> SPMSATALLQKA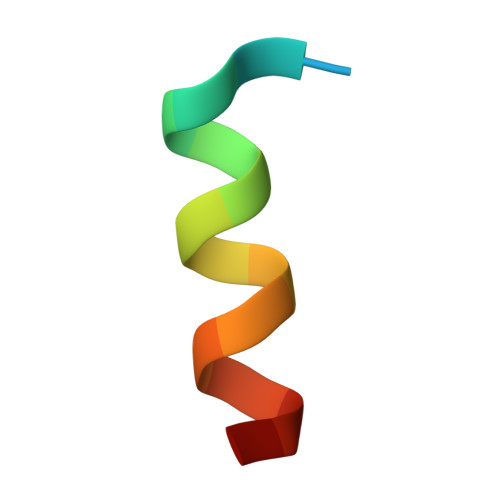AQMGS>LMSDWEDEDLDTDNDNIPDSYERNGYTIKDLIAVKWEDSFAEQGYKKYVSNYLESNTAGDPYTDYEKASGSFDKAIKTEARDPLVAAYPIVGVGMEKLIISTNEHASTDQGKTVSRATTNSKTESNTAGVSVNVGYQNGFTANVTTNYSHTTDNSTAVQDSNGESWNTGLSINKGESAYINANVRYYNTGTAPMYKVTPTTNLVLDGDTLSTIKAQENQIGNNLSPGDTYPKKGLSPLALNTMDQFSSRLIPINYDQLKKLDAGKQIKLETTQVSGNFGTKNSSGQIVTEGNSWSDYISQIDSISASIILDTENESYERRVTAKNLQDPEDKTPELTIGEAIEKAFGATKKDGLLYFNDIPIDESCVELIFDDNTANKIKDSLKTLSDKKIYNVKLERGMNILIKTPTYFTNFDDYNNYPSTWSNVNTTNQDGLQGSANKLNGETKIKIPMSELKPYKRYVFSGYSKDPLTSNSIIVKIKAKEEKTDYLVPEQGYTKFSYEFETTEKDSSNIEITLIGSGTTYLDNLSITELNSTPEILDEPEVK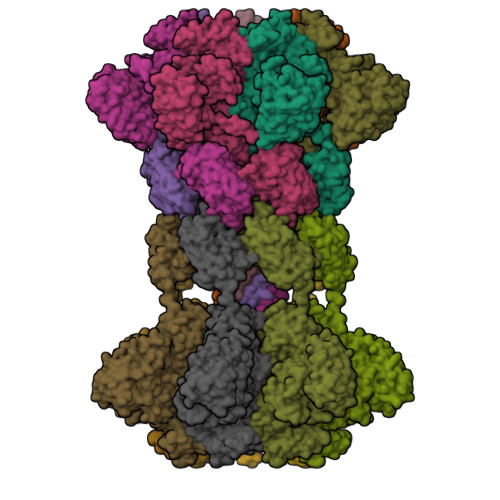IPTDQEIMDAHKIYFADLNFNPSTGNTYINGMYFAPTQTNKEALDYIQKYRVEATLQYSGFKDIGTKDKEMRNYLGDPNQPKTNYVNLRSYFTGGENIMTYKKLRIYAITPDDRELLVLSVD[14x]Proline racemase of Trypanosoma cruzi (TcPRAC) is an enzyme present at all stages of the parasite life cycle, contributing to immune escape and persistence of the parasite in the host. Gene over-expression increases virulence, while knockdown appears lethal for T. cruzi. The structure also showed that TcPRAC crystallizes as a homodimer and bears a catalytic site on each subunit.

Atoms C2 and C5 of BrOxoPA are covalently bound to the sulfur atoms of Cys300 and Cys130, respectively. These covalent interactions can explain the irreversible inhibition of TcPRAC by BrOxoPA. The carboxylate moiety of the inhibitor also forms a hydrogen-bonding network with the main polypeptide chain or side chains of Gly131, His132, Gly301, and Thr302 in the active site region. No electron density was observed for the bromine atom of the BrOxoPA inhibitor in difference Fourier maps, and X-ray fluorescence scans indicate the absence of bromine in crystals of the complex, suggesting that the bromine atom of the inhibitor was cleaved during the binding reaction of BrOxoPA with the enzyme. The crystal structure with BrOxoPA shows an enantioselective addition, 2S, at C2, while C3 remains achiral. The BrOxoPA complex also shows that a second reaction took place, leading to a very tightly bound complex, as indicated by the cavity volume. The saturation of C2 allows the folding of the molecule to position C5 and its bromine atom close to Cys130. The second attack released the bromine atom as reported for haloketones. The complex with BrOxoPA, which formed two bonds within each site, displayed the smallest volumes. Indeed, alpha-bromoketones, as found in BrOxoPA, are known to be highly reactive.

>MGQEKLLFDQKYKIIKGEKKEKKKNQRANRREHQQKREIMRFKKSFTCIDMHTEGEAARIVTSGLPHIPGSNMAEKKAYLQENMDYLRRGIMLEPRGHDDMFGAFLFDPIEEGADLGIVFMDTGGYLNMCGHNSIAAVTAAVETGIVSVPAKATNVPVVLDTPAGLVRGTAHLQSGTESEVSNASIINVPSFLYQQDVVVVLPKPYGEVRVDIAFGGNFFAIVPAEQLGIDISVQNLSRLQEAGELLRTEINRSVKVQHPQLPHINTVDCVEIYGPPTNPEANYKNVVIFGNRQADRSPCGTGTSAKMATLYAKGQLRIGETFVYESILGSLFQGRVLGEERIPGVKVPVTKDAEEGMLVVTAEITGKAFIMGFNTMLFDPTDPFKNGFTLKQYIWSSSVDKLAAALEHHHHHH[2x]>MLEVVTAGEPLVALVPQEPGHLRGKRLLEVYVGGAEVNVAVALARLGVKVGFVGRVGEDELGAMVEERLRAEGVDLTHFRRAPGFTGLYLREYLPLGQGRVFYYRKGSAGSALAPGAFDPDYLEGVRFLHLSGITPALSPEARAFSLWAMEEAKRRGVRVSLDVNYRQTLWSPEEARGFLERALPGVDLLFLSEEEAELLFGRVEEALRALSAPEVVLKRGAKGAWAFVDGRRVEGSAFAVEAVDPVGAGDAFAAGYLAGAVWGLPVEERLRLANLLGASVAASRGDHEGAPYREDLEVLLKATQTFMR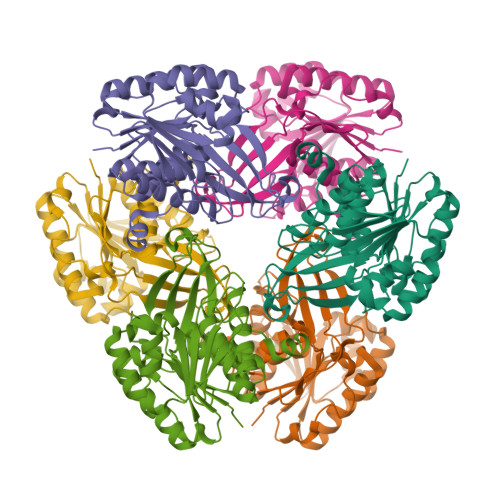[6x]>[2x]GM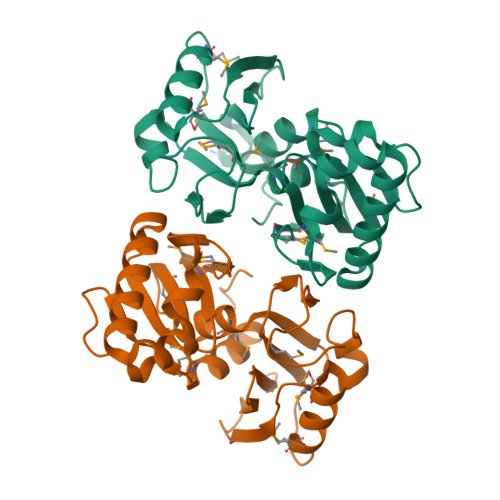AEDQTVLAIDIGGSHVKIGLSTDGEERKVESGKTMTGPEMVAAVTAMAKDMTYDVIAMGYPGPVVHNKPLREPVNLGEGWVGYDYEGAFGRPVRIVNDALMQAIGSYNGGRMLFLGLGTGLGAAMIVENVAQPMEIAHLPYRKGKTYEHYVSEAYREKKGNAKWQKRVQDVVERLSAALEPDEVVIGGGNVERLENLPPKCRRGDNAMAFEGGFRLWKNADLIV>[2x]MANPYERGPDPTESSIEAVRGPFAVAQTTVSRLQADGFGGGTIYYPTDTSQGTFGAVAISPGFTAGQESIAWLGPRIASQGFVVITIDTITRLDQPDSRGRQLQAALDHLRTNSVVRNRIDPNRMAVMGHSMGGGGALSAAANNTSLEAAIPLQGWHTRKNWSSVRTPTLVVGAQLDTIAPVSSHSEAFYNSLPSDLDKAYMELRGASHLVSNTPDTTTAKYSIAWLKRFVDDDLRYEQFLCPAPDDFAISEYRSTCPFLEHHHHHH

Herein, we report a novel polyester hydrolase (PHL7), isolated from plant composts with a high efficiency to degrade amorphous PET films and post‐consumer PET thermoform packaging. All of them contained the GXSXG box, a conserved Ser‐Asp‐His triad and an alpha/beta‐hydrolase fold. The polyester hydrolase PHL7, isolated from a compost metagenome, completely hydrolyzes amorphous PET films, releasing 91 mg of terephthalic acid per hour and mg of enzyme. Structural analysis of the enzyme indicated that leucine at position 210 contributed to the high PET hydrolytic activity compared to other polyester hydrolases.

PHL7 has a leucine at position 210, whereas other known type I polyester hydrolases harbor a phenylalanine. To explore the reason for the considerably higher activity of PHL7, we exchanged leucine 210 in PHL7 with phenylalanine. As a result, the activity of the variant dropped to the level of PHL3. Residues G62, T64, S69, H130, S131, M132, W156, D177, A180, H209, N213 (catalytic triad in italic) are conserved between PHL7 and LCC, whereas F63 (LCC: Y95), L93 (F125), Q95 (Y127), I179 (V212) differed. Figure 2A also shows that the active site pocket of PHL7 is more open than that of LCC. However, the plasticity of these predominantly hydrophobic regions near the active site may contribute to binding of larger PET substrates and be a key for a more tolerant recognition and effective processing of PET at elevated temperatures concomitant with increased polymer chain mobility. The crystal structure of PHL7 shows a metal ion coordinated by the side chains of Glu148 and Asp233, the carbonyl group of Phe230 and three water molecules in a distorted octahedral geometry. We modeled this ion as sodium due to the electron density at this position and the high concentration (100 mm) of Na+ in the crystallization buffer.> AVTCPTGQTTANEACCVLFPVIDLLQEELFDGGECGEEAHAALRLAFHDAIGFSKNGGKGGGADGSILAFHQTETTYAANSGIEDIITAQLPIFQKTNLTAGDFVHLAAAIGTGNCPGSPQLAYSFGRPPPVAPAPDGTVPEPTDSVTDILARFSEAGFVTAEVIWLLASHSIAAASKIDTSAPRTPFDSTPALFDTQFYLETILNGTLLPGDGGAHTGEVLSPIAGEMRLQSDFAFAQDPRTACLWQEPINDQAFIQGKFFAAMKKLQVLGQTGLTDCSDVIPVPASLPGPITFPAGFSEADVISACTATPLPSLATIAGPKPTIPPVPL

Here, we characterize a similar enzyme (ApeLiP) from a fungus of the order Agaricales (with ~13,000 described species), the soil-inhabiting mushroom Agrocybe pediades. X-ray crystallography revealed that ApeLiP is structurally related to Polyporales LiPs, with a conserved heme-pocket and a solvent-exposed tryptophan. Its biochemical characterization shows that ApeLiP can oxidize both phenolic and non-phenolic lignin model-compounds, as well as different dyes. Moreover, using stopped-flow rapid spectrophotometry and 2D-NMR, we demonstrate that ApeLiP can also act on real lignin. Characterization of a variant lacking the above tryptophan residue shows that this is the oxidation site for lignin and other high redox-potential substrates, and also plays a role in phenolic substrate oxidation.

ApeLiP was successfully crystallized in the orthorhombic P212121 space group containing one molecule in the asymmetric unit. Its structure was determined by molecular replacement, and refined against the 1.85 Å diffraction data. It consists of 331 residues (from Thr1 of the mature protein to Leu331, only lacking the C-terminal Arg332) and contains one heme molecule, two Ca2+ ions and two Zn2+ ions. The overall folding is mainly helical, with 14 α-helices, and one short antiparallel β-sheet. Four disulfide bridges (Cys4-Cys16, Cys15-Cys279, Cys35-Cys116 and Cys245-Cys308) contribute to maintain the protein conformation together with the above Ca2+ ions, which are coordinated by Asp49, Gly63, Asp64 and Ser66 (Ca2+ at the heme distal side) and by Ser172, Asp196, Thr191, Leu194 and Asp189 (Ca2+ at the heme proximal side). Moreover, the presence of two structural zinc ions on the protein surface, from the crystallization medium, contributed to the folding stability. The heme pocket also includes conserved Phe188 and Asp234 on the proximal side, along with Phe47, His48 and Arg44 on the distal side, the two latter putatively involved in heme peroxidase activation by H2O2. The second channel is smaller and appears located directly on the heme propionates, occupying a position equivalent to that of the Mn2+-binding site in MnP and VP enzymes. However, the Glu37/Ala41/Ser177 residues identified at the ApeLiP channel are not compatible with cation coordination. The crystal structure also presents a solvent exposed tryptophan (Trp166), as the one reported for oxidation of bulky and high redox-potential aromatic substrates including the lignin molecule.> MSQRITIDPVTRIEGHLRIDCE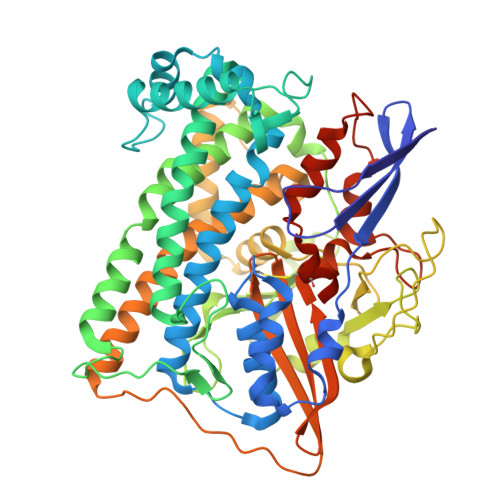IENGVVSKAWASGTMWRGMEEIVKNRDPRDAWMIVQRICGVCTTTHALSSVRAAESALNIDVPVNAQYIRNIILAAHTTHDHIVHFYQLSALDWVDITSALQADPTKASEMLKGVSTWHLNSPEEFTKVQNKIKDLVASGQLGIFANGYWGHPAMKLPPEVNLIAVAHYLQALESQRDANRVVALLGGKTPHIQNLAVGGVANPINLDGLGVLNLERLMYIKSFIDKLSDFVEQVYKVDTAVIAAFYPEWLTRGKGAVNYLSVPEFPTDSKNGSFLFPGGYIENADLSSYRPITSHSDEYLIKGIQESAKHSWYKDEAPQAPWEGTTIPAYDGWSDDGKYSWVKSPTFYGKTVEVGPLANMLVKLAAGRESTQNKLNEIVAIYQKLTGNTLEVAQLHSTLGRIIGRTVHSSELQDILQNQYSALITNIGKGDHTTFVKPNIPATGEFKGVGFLEAPRGMLSHWMVIKDGIISNYQAVVPSTWNSGPRNFNDDVGPYEQSLVGTPVADPNKPLEVVRTIHSFDPCMACAVHVVDADGNEVVSVKVL> MLMRPLDLTEKRGKKVTIYFEGKELEAYEGEKLPVALLANEIYWLTTSNEGRKRGAFTFGPVPMTVNGVKGLEARRIKVKDGMKIERQGYYDFHEEPVVEPGEIERVVVDVAIIGGGPAGIGAALELQQYLTVALIEERGWLGGDMWLKGIKQEGFNKDSRKVVEELVGKLNENTKIYLETSALGVFDKGEYFLVPVVRGDKLIEILAKRVVLATGAIDSTMLFENNDMPGVFRRDFALEVMNVWEVAPGRKVAVTGSKADEVIQELERWGIDYVHIPNVKRVEGNEKVERVIDMNNHEYKVDALIFADGRRPDINPITQAGGKLRFRRGYYSPVLDEYHRIKDGIYVAGSAVSIKPHYANYLEGKLVGAYILKEFGYDAQPCIYEEKLREYEPESLSIPRIPLDKFNLEDVQICGCDVSLKKVDEVIRKGITDLQIIKRLTHLAMGFCQGRYCLFNG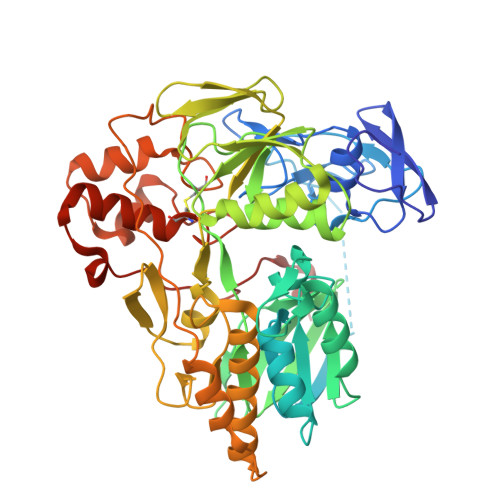AVVVSQRTGKKLSEIDLPVARSPIKNVKMGILARR> MRGSHHHHHHGSMPFEIVFEGAKEFAQLIETASRLIDEAAFKVTEEGISMRAMDPSRVVLIDLNLPASIFSKYEVDGEETIGVNMDHLKKVLKRGKAKETLILRKGEENFLEISLQGTATRTFKLPLIDVEEIEVDLPELPFTAKVVILGDVIKEAVKDASLVSDSMKFIAKENEFTMRAEGETQEVEVKLTLEDEGLLDIEVQEETKSAYGISYLSDMVKGLGKADEVTIKFGNEMPMQMEYYIRDEGRLIFLLAPRVEE

The bacterial sliding clamp is referred to as the β clamp, whereas the eukaryotic and archaeal sliding clamp protein is called the proliferative cell nuclear antigen (PCNA). Clamps are constructed from either two (β) or three monomers (PCNA) to yield a ring composed of six domains, which share similar protein folds. Hence, across every domain of life, the extraordinary efficacy of the replicative polymerase complex is dependent on their interaction with sliding clamps, which encircle DNA and greatly enhance their processivity. We have shown that PolD uses two distinct PIP-boxes for molecular recognition of PCNA, which are located in the C-terminal region of their DP2 subunit.

In the peripheral region of the complex, the DP2 KH domain, the DP1 OB domain, and some regions of the PCNA were found to be flexible and the local resolution map ranged between 4.0 and 6.0 Å. In these regions, crystal structures of PolD DP1 (144–619) and DP2 (1–1050) individual subunits, and the structure of the P. abyssi PCNA (from this study using X-ray crystallography at 2.3 Å resolution) were used in model building. The structure of PCNA in the complex is not distorted compared with the structure of free PCNA and we conclude that the cryo-EM structure represents a stable interaction of DNA-bound PolD with a closed PCNA clamp.>MSKLSVFFIFLFCSIATAAESLPDLKIEKLDEGVYVHTSFEEVNGWGVVPKHGLVVLVNAEAYLIDTPFTAKDTEKLVTWFVERGYKIKGSISSHFHSDSTGGIEWLNSRSIPTYASELTNELLKKDGKVQATNSFSGVNYWLVKNKIEV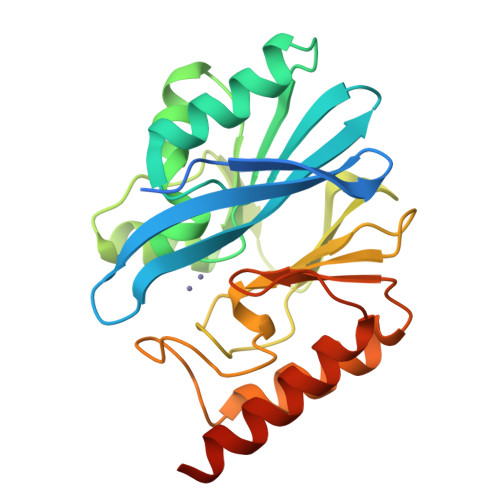FYPGPGHTPDNVVVWLPERKILFGGCFIKPYGLGNLGDANIEAWPKSAKLLKSKYGKAKLVVPGHSEVGDASLLKLTLEQAVKGLNESKKPSKPSN[4x]>[4x]MRKIGIIGGTFDPPHYGHLLIANEVYHALNLEEVWFLPNQIPPHKQGRDITSVESRLQMLELATEAEEHFSICLEELSRKG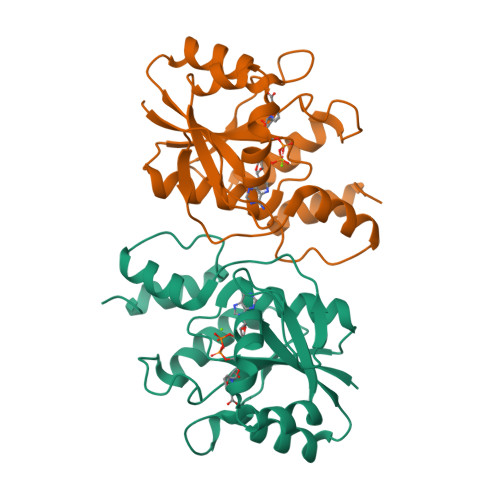PSYTYDTMLQLTKKYPDVQFHFIIGGDMVEYLPKWYNIEALLDLVTFVGVARPGYKLRTPYPITTVEIPEFAVSSSLLRERYKEKKTCKYLLPEKVQVYIERNGLYES> MPEITRRRALTAAAAVAATASAAVTLAAPAASAAGHHEPAAPESFDEVYKGRRIQGRPAGGGAHHHEHGGGYEVFVDGVQLHVLRNADGSWISVVSHYDPVPTPRAAARAAVDEL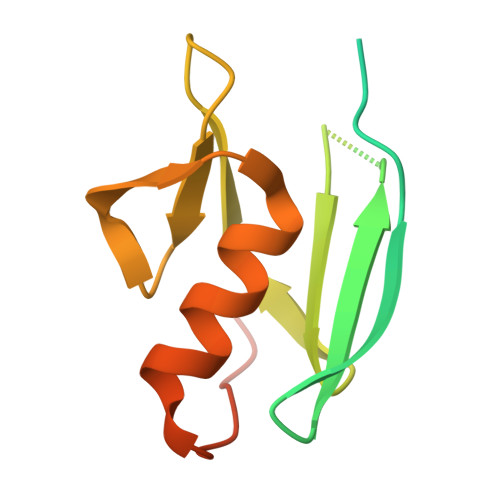QGAPLLPFPANLEHHHHHH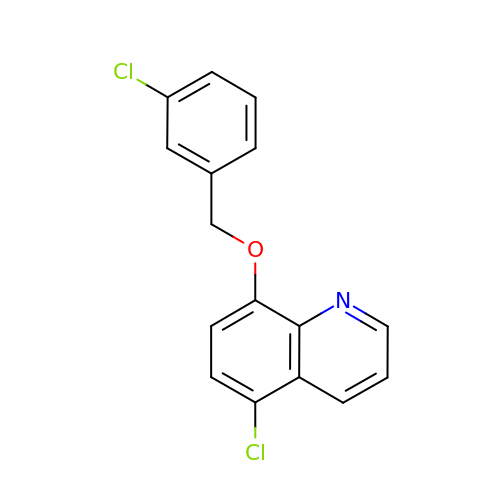5-chloro-8-[(3-chlorobenzyl)oxy]quinoline | C16 H11 Cl2 N O | BIHPUIBBWFPTCY-UHFFFAOYSA-N> IVGGQECKDGECPWQALLINEENEGFCGGTILSEFYILT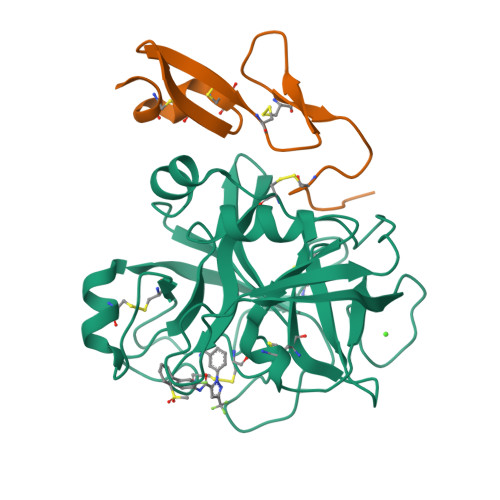AAHCLYQAKRFKVRVGDRNTEQEEGGEAVHEVEVVIKHNRFTKETYDFDIAVLRLKTPITFRMNVAPACLPERDWAESTLMTQKTGIVSGFGRTHEKGRQSTRLKMLEVPYVDRNSCKLSSSFIITQNMFCAGYDTKQEDACQGDSGGPHVTRFKDTYFVTGIVSWGEGCARKGKYGIYTKVTAFLKWIDRSMKT;> KLCSLDNGDCDQFCHEEQNSVVCSCARGYTLADNGKACIPTGPYPCGKQTLE>[4x]KTTYERTFVKKDAETKEVLEGAGFKISNSDGKFLKLTDKDGQSVSIGEGFIDVLA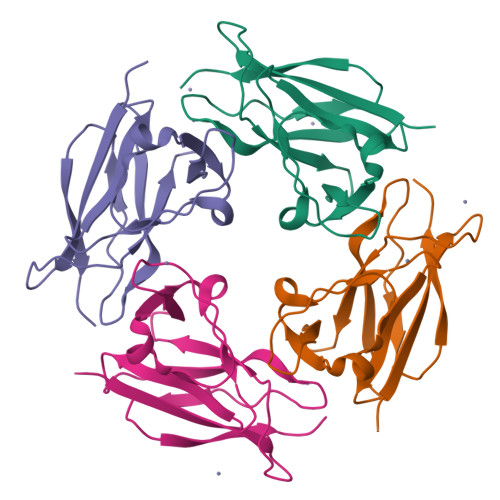NNYRLTWVAESDATVFTSDKSGKFGLNGFADNTTTYTAVETNVPDGYDAAANTDFKADNSSSDILDAPSGILPLEHHHHHH>MRKAVSQRNKLILWTRGGGRCYLCNCALLGDLISGKDKLNKGYIAHIVAAEIDGPRGDPIRSPLLCDDVENLILLCDAHHRLIDVEAVAEYSEPRLQQIKRAHEARVEAVTEITADRGTHMLFYSARIGEHDCPIQAQDARSAVLPAYYPKDRHPIALDVARSEYADNEAQYWQFQIENLNRQFERKVRPLLADGHIDHLSVFGLAPQPLLIHLGRLLSDLRKVRVHQLHREPKGWDWRNERPPVVYKTDRTGHGRTIALKIGISATIVDERITRCLGEDTTIWSLSAEGAHNDILHSEGDLQTFRSTCRRLFDAIKAAHPDATDLHIFPAMPVSTAIELGRIWMPKADLPL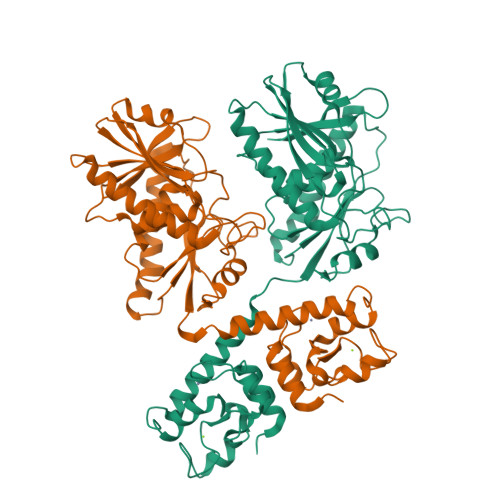HIYDENRTAGGFFHRHSLGGVSIPKTEEPIYG[2x]In contrast, CBA120 contained multiple genes for putative TSPs (TSP1-TSP4), genes that are more commonly associated with Podoviridae rather than Myoviridae. Analytical gel filtration of purified TSP1 revealed a single homogeneous peak at ∼252 kDa based on regression analysis of gel filtration standards (data not shown), suggesting that similar to all other tailspike proteins with known structures, TSP1 forms a trimer in solution (predicted 82 kDa monomer, 246 kDa trimer). The TSP1 trimer assumes an elongated rod-like shape of approximately 170 Å in length and 75 Å in diameter at the widest region.

To identify possible sugar binding sites, the crystals were flash soaked in high concentrations of readily available mono-saccharides (mannose and glucose) and di-saccharides (α-lactose and α-maltose). Of these, binding sites of glucose, α-lactose, and maltose were evident in the difference electron density maps. All glucose molecules exhibit the β conformation. The binding site is located at the periphery of the hole generated by the D3-D4 intervening region, adjacent to subdomain D4. The glucose engages a single subunit and the interactions include both direct hydrogen bonds to the protein ligand-water-protein bridged hydrogen bonds: The carboxylate group of Glu639 forms a hydrogen bond with the C1 hydroxyl group. The amine group of Lys662 forms hydrogen bonds with both the C1 and C2 hydroxyl groups. The backbone amide of Lys615 is hydrogen bonded to the primary alcohol hydroxyl group of C6. A water mediated interaction bridges the backbone carbonyl of Glu639 and the C6 hydroxyl group. A second water molecule bridges the backbone amide of Glu639 and the hemiacetal oxygen atom of the glucose. The sugar-binding sites this study identified are located remotely from the proposed catalytic site, suggesting that TSP1 acts on a glycosidic bond connecting different saccharide units.

>[3x]MNEMFSQGGKGSTGILTNKQAVARHFGVKQSEVVYFSVGVDLGGYKVIYDKETQRAYSLPVGIASGTTAVSLSTAAVLVHSAGSVDLGSLAVSREEYVTLPGSFDSGSTLNVKNELLTYTDGKYRWDGILPKTVAPGSTPASTGGVGLGAWISVGDASLRTQLANGDGSLIGIHPQGTLNNVLTVRTPEQYNAVGDGIADDTSKLKEMLSDINNVPETLPDAAAVNSYMEQVAVKIDLTKLYRFTETLYIPPGVSIEIPTSNFFTRECKQGLFYDPVDKNTAAISLMVYRKQPDGSYKLNKDVDYYPTGLDIDNGDAITCARKIDINNLNLITAPGVKVGVKWIGGAGCTTKGLSIGENTGSDITTARLPRVGLLQSASWGSIHENLRILYKTQGAVFIDSNGGAAVNNAYISRLGNTNGELEQAVYKPAGFTEVGDVAVTQFAGSEVKFNSPIIEQASFDFVHAGRDTDSYGLFMVDKPHIESSGGKKKHSFYLINTSSNVTLSGVGLSGQDPDLDSMYFLKNCPETARNVVRGQMPISGVKLVRGTGNYPTLVLDCTNMGSQFQFGEVGDIFYIKDVVGVKADTLYIDPVNGNNYNWGTNGTKPIRELTNIAKICQLFRCKSVYLNAGESVITSNTELPMVVFEGPGSLKANSGSSFLIKAGGTLSLIGLSGISTDGGHMFRVSTVEKVNIHTNCSVNAGAAYVVLSEVQGNIEYRQLFYSVNCSKYIGATAGQTIAGIMVKTATRPTGIDAAPVDGNVSLTYKIIESHHHHHH>[4x]PQFEKIEGRMIRILYLLVKPESMSHEQFRKECVVHFQMSAGMPGLHKYEVRLVAGNPTDTHVPYLDVGRIDAIGECWFASEEQYQVYMESD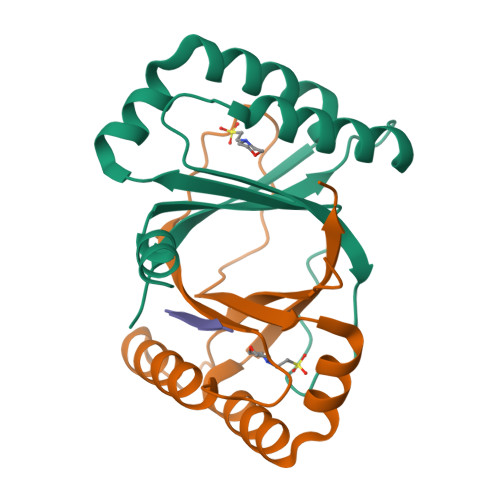IRKAWFEHGKYFIGQLKPFVTEELV;>[2x]ASWSA>[5x]APQSITELCSEYHNTQIYTINDKILSYTESMAGKREMVIITFKSGATFQVEVPGSQHIDSQKKAIERMKD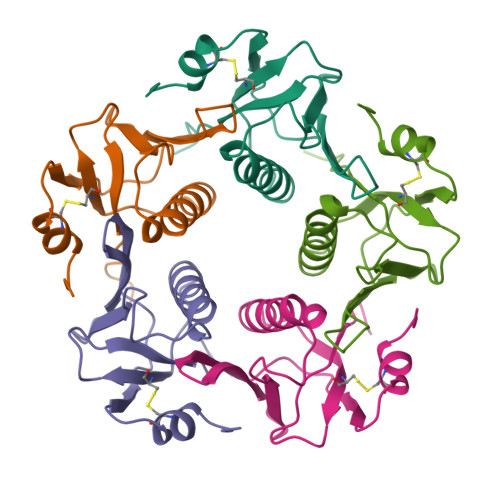TLRITYLTETKIDKLCVWNNKTPNSIAAISMEKLAGFGAVGAGATAEETRMLHAFDTLA> MKSIKIIVLGSALALLVGGCFVGSRDPNETRYPKAPMPLQNQTST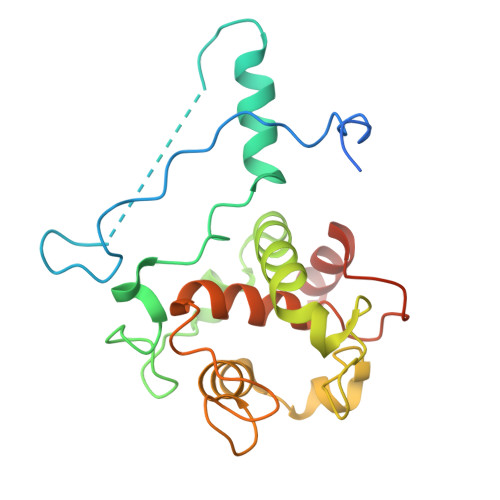LKTAEEIRRESVAQNTPGAREAAALRDRVTPLNLQQVNEQDVAGNDPLGSPARVVLDEGEMYRDPVEIYREGRALFQNNCVGCHGHNGCGNVPRSTNFTDPGWQENNSDGGIYSSIYNGKGIGNGGGAMPAYYNQLSPQQIRYLVAYLRAFKGRQCNGLPTLSDVERMVAERQNKP>[2x]MVLPDIKKGKDMINILPFEIISRNTKTLLITYISSVDITHEGMKKVLESLRSKQGIISEYLLDKLLDESLIDKDKGKEFLITTGVINKTKTSPLWVNSVIISDVPHLFSNAREQWKCDGVFVSHIIDIKDNNINVSDSTLIWLHLENYHSDIVKRIYSKFESNPGVAFIQSYYLKESFRIDGVYSPDLGTPCHFCHIERWLSREEKSFRRNEMSWANLLQLLKKYQMTLPALALGESERGFSYHLIKRRLQELTGTSLVKSHVDNFMSSVSADLITCILCKEPVIHWQACSCLER;> MGHHHHHHMELKASEFGVVLSVDALKLSRQSPLGVGIGGGGGGGGGGSCGGQGGGCGGCSNGCSGGNGGSGGSGSHI;> MSKHELSLVEVTHYTDPEVLAIVKDFHVRGNFASLPEFAERTFVSAVPLAHLEKFENKEVLFRPGFSSVINISSSHNFSRERLPSGINFCDKNKLSIRTIEKLLVNAFSSP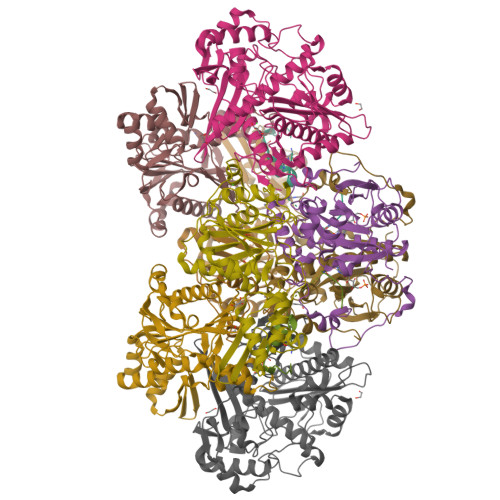DPGSVRRPYPSGGALYPIEVFLCRLSENTENWQAGTNVYHYLPLSQALEPVATCNTQSLYRSLSGGDSERLGKPHFALVYCIIFEKALFKYRYRGYRMALMETGSMYQNAVLVADQIGLKNRVWAGYTDSYVAKTMNLDQRTVAPLIVQFFGDVNDDKCLQ;> MINVYSNLMSAWPATMAMSPKLNRNMPTFSQIWDYERITPASAAGETLKSIQGAIGEYFERRHFFNEIVTGGQKTLYEMMPPSAAKAFTEAFFQISSLTRDEIITHKFKTVRAFNLFSLEQQEIPAVIIALDNITAADDLKFYPDRDTCGCSFHGSLNDAIEGSLCEFMERQSLLLYWLQGKANTEISSEIVTGINHIDEILLALRSEGDIRIFDITLPGAPGHAVLTLYGTKNKISRIKYSTGLSYANSLKKALCKSVVELWQSYICLHNFLIGGYTDDDIIDSYQRHFMSCNKYESFTDLCENTVLLSDDVKLTLEENITSDTNLLNYLQQISDNIFVYYARERVSNSLVWYTKIVSPDFFLHMNNSGAININNKIYHTGDGIKVRESKMVPFP>HHHHHHFNLPPGNYKKPVLLYSSNGGHFLRILPDGTVDGTRDRSDQHIQLQLSAESVGEVYIKSTETGQYLAMDTDGLLYGS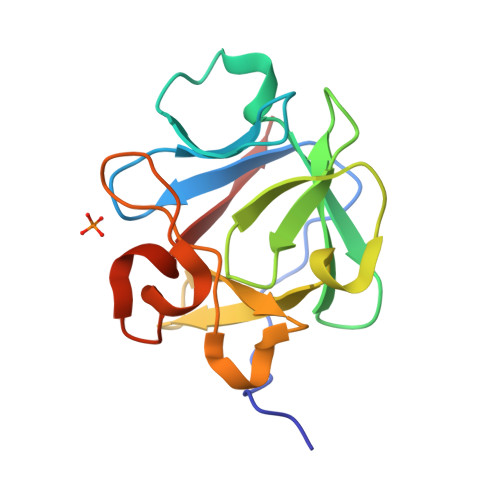QTPNEECLFLERLEENHYNTYISKKHAEKNWFVGLKKNGSVKRGPRTHYGQKAILFLVLPVSSD[2x]> SMSRSGTDPQQRQQASEADAAYTPFLANDHQHIRYNPLQDEWVLVSAHRMKRPWQGQVEPQLLKTVPRHDPLNPLCPGAIRANGEVNPQYDSTFLFDNDFPALQPDAPSPGPSDHPLFQAKSARGVCKVMCFHPWSDVTLPLMSVPEIRAVVDAWASVTEELGAQYPWVQIFENKGAMMGCSNPHPHCQVWASSFLPDIAQREERSQQAYKSQHGEPLLMEYSRQELLRKERLVLTSEHWLVLVPFWATWPYQTLLLPRRH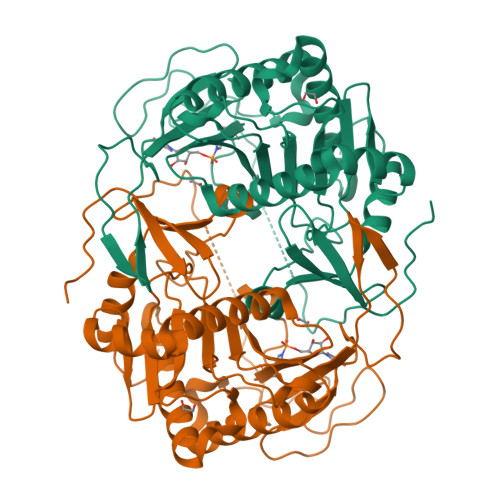VRRLPELTPAERDDLASIMKKLLTKYDNLFETSFPYSMGWHGAPTGSEAGANWDHWQLHAHYYPPLLRSATVRKFMVGYEMLAQAQRDLTPEQAAERLRALPEVHYHLGQKDRETATIA> GHMASATARVRIYPLALAKVVKHAASSLQREVAGLLVGKSAGKVLEIWDAVTGEQYGTPAYVQLDEMVMAK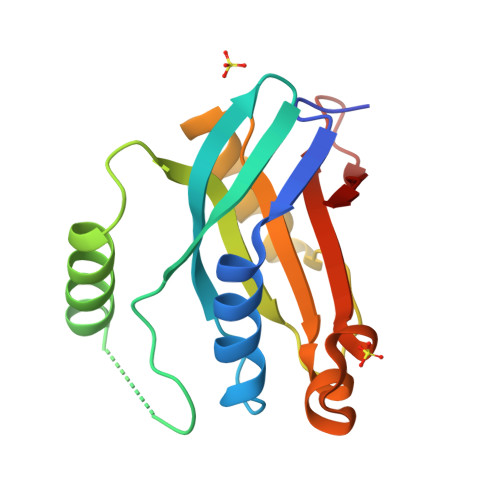VAEELSKSDKNLYIVGWYHSHPGLDVFLSPTDIDTQKRYQAMFSKAVALVVDPVDYAKTRRISSLKFKVFQISKEGRVVSLPVS>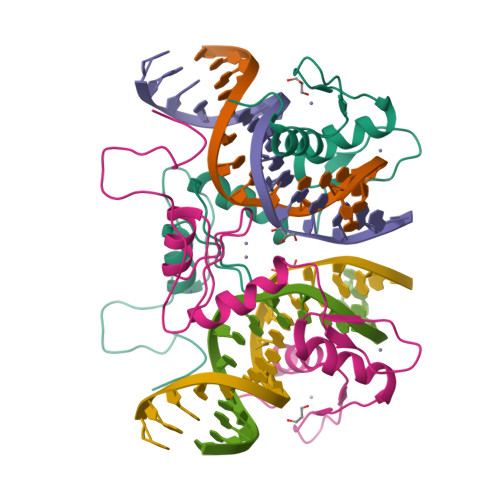 GSVEEKEEEEEEEENEEEECAAYQCNMEGCTMSFSSEKQLMLHKRNICPIKGCGKNFFSHKYLVQHQRVHSDDRPLKCPWKGCKMTFKWAWSRTEHIRVHTGARPYVCAEPDCGQTFRFVSDFSRHKRKTGHSVKKTNKR> TRSNENRIKLVPIAPSRGIIYDRNGIPLALNRTIYQIEMMPEKVDNVQQTLDALRSVVDLTDDDIAAF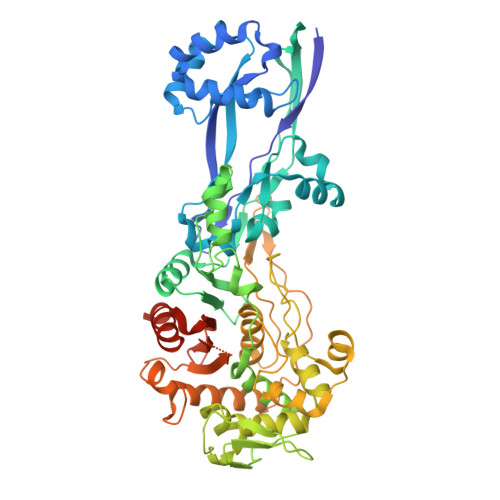RKERARSHRFTSIPVKTNLTEVQVARFAVNQYRFPGVEVKGYKRRYYPYGSALTHVIGYVSKINDKDVERLNNDGKLANYAATHDIGKLGIERYYEDVLHGQTGYEEVEVNNRGRVIRQLKEVPPQAGHDIYLTLDLKLQQYIETLLAGSRAAVVVTDPRTGGVLALVSTPSYDPNLFVDGISSKDYSALLNDPNTPLVNRATQGVYPPASTVKPYVAVSALSAGVITRNTTLFDPGWWQLPGSEKRYRDWKKWGHGRLNVTRSLEESADTFFYQVAYDMGIDRLSEWMGKFGYGHYTGIDLAEERSGNMPTREWKQKRFKKPWYQGDTIPVGIGQGYWTATPIQMSKALMILINDGIVKVPHLLMSTAEDGKQVPWVQPHEPPVGDIHSGYWELAKDGMYGVANRPNGTAHKYFASAPYKIAAKSGTAQVFGLKANETYNAHKIAERLRDHKLMTAFAPYNNPQVAVAMILENGGAGPAVGTLMRQILDHIMLGDNNTDLPAENPAVAAAEDH>NNAGAC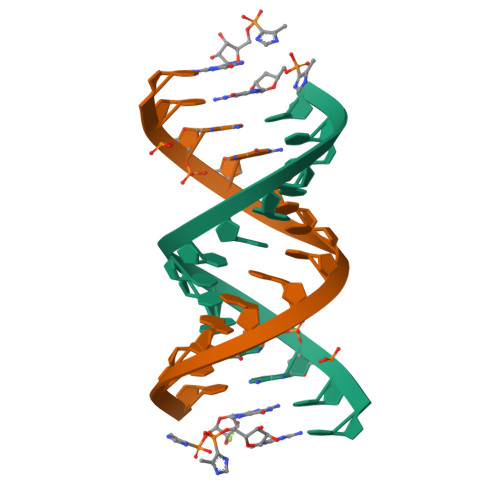UUAAGUCU[2x]>[2x]GSKGPLDQLEKGGETAQSADPQWEQLNNKNLSMPLLPADFHKENTVTNDWIPEGEEDDDYLDLEKIFSEDDDYIDIVDSLSVSPTDSDVSAGNILQLFHGKSRIQRLNILNAKFAFNLYRVLKDQVNTFDNIFIAPVGISTAMGMISLGLKGETHEQVHSILHFKDFVNASSKYEITTIHNLF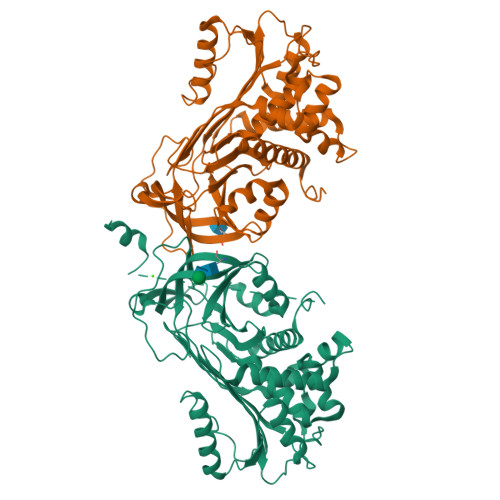RKLTHRLFRRNFGYTLRSVNDLYIQKQFPILLDFKTKVREYYFAEAQIADFSDPAFISKTNNHIMKLTKGLIKDALENIDPATQMMILNCIYFKGSWVNKFPVEMTHNHNFRLNEREVVKVSMMQTKGNFLAANDQELDCDILQLEYVGGISMLIVVPHKMSGMKTLEAQLTPRVVERWQKSMTNRTREVLLPKFKLEKNYNLVESLKLMGIRMLFDKNGNMAGISDQRIAIDLFKHQGTITVNEEGTQATTVTTVGFMPLSTQVRFTVDRPFLFLIYEHRTSCLLFMGRVANPSRS> UUGGGCCGGCGGCGGGUCC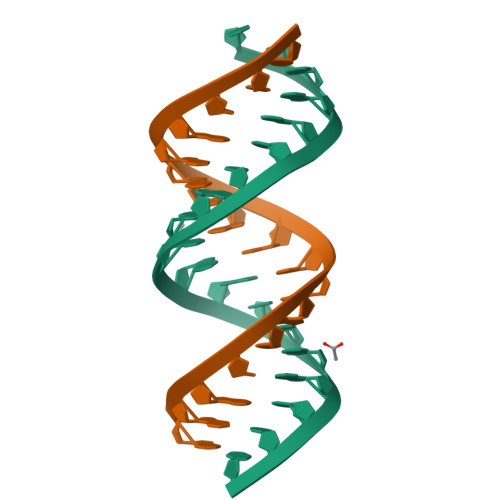;> GGGCCGGCGGCGGGUCC>APLLKTLPFLAAAYAAELDLPNFSALNRRQDNSTSSSAGCSLDQTVAPGNLTLCGNATLFTTFRPKARFIAPEGWMNAPMGLYQRADGSIHAGYQSHPKHIQWGNISQGAAYSSDFTSWTDFNGSEGYKTIWPSQIYDIRGVFDGSIIKEGIDGYPTILYTSTSFGPLGATLNEAEGTETQSLAYTTDDGASWIKLGYGAGQNPVIYEWPETNLTGFRDPYVFQSPRLEALLANTTSITNATGDHFATISGGVHGDGARLFLYRQHTTGEFIKWTYLGPLVTTGYKESYGEWSGNYGINFETAGVTRLNPAGAAWDNGSDTTAVDFVTFGTEQGRADHQNHWPLWAAVDYEVRDNGSIEAVIAYSGVQDWGRSYAYASFPVEGYRQVSVGWIYEDDDNVILAKQFGYQGAFTLFRDLFVKVVENVSPSTPGLFEQASWSTKNSTDGMSVTVTTLGQRVVPETLAAYKGNSTVSTLAPVMLNESAAAYTPFSSQPTDRFYALTGSFEFGLNTTAKAGFRVLASEEEYTDIWFDPASENLTVVRTASSLIKSFGNDTELAKVKLYEIVGAESKTLNLTVFVDGSVIEIYANDEVALSTRAYPWLANST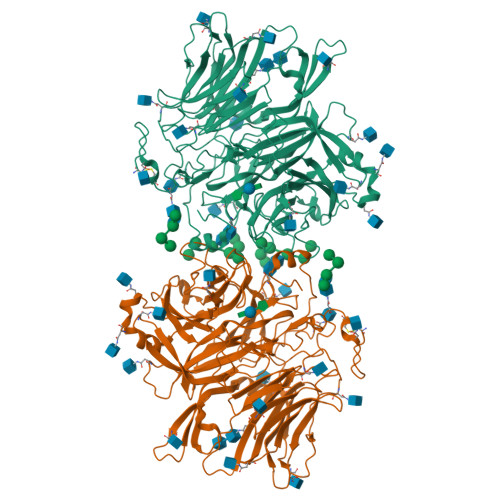GAGLLADGTTAGDVVGVSGLELWDGLVDAWPARPANTSQGLVWDGPTAAMYGLFAGY[2x]> GAMGSGEPQSPSRRVFNPYTEFKEFSRKQIKDMEKMFKQYDAGRDGFIDLMALKLMMEKLGAPQTHLGLKNMIKEVDEDFDSKLSFREFLLIFRKAAAGELQEDSGLCVLAR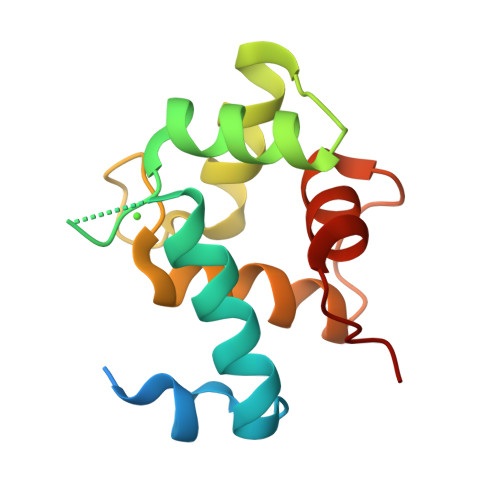LSEIDVSS> GNYALGPEGLKKALAETGSHILVMDLYAKTMIKQPNVNLSNIDLGSEGGELLKNIHLNQELSRINANYWLDTAKPQIQKTARNIVNYDEQFQNYYDTLVETVQKKDKAGLK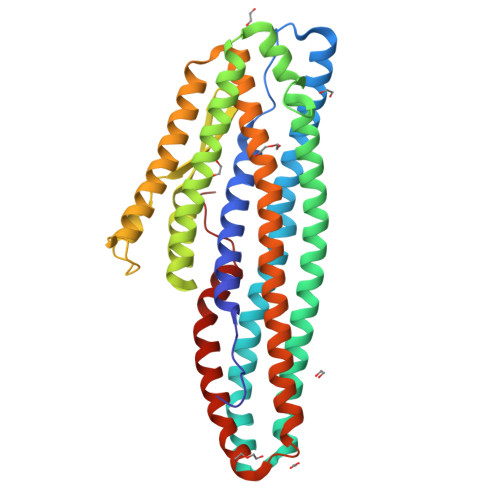EGINDLITTINTNSKEVTDVIKMLQDFKGKLYQNSTDFKNNVGGPDGKGGLTAILAGQQATIPQLQAEIEQLRSTQKKHFDDVLAWSIGGGLGAAILVIAAIGGAVVIVVTGGTATPAVVGGLSALGAAGIGLGTAAGVTASKHMDSYNEISNKIGELSMKADRANQAVLSLTNAKETLAYLYQTVDQAILSLTNIQKQWNTMGANYTDLLDNIDSMQDHKFSLIPDDLKAAKESWNDIHKDAEFISKDIAFKQ> 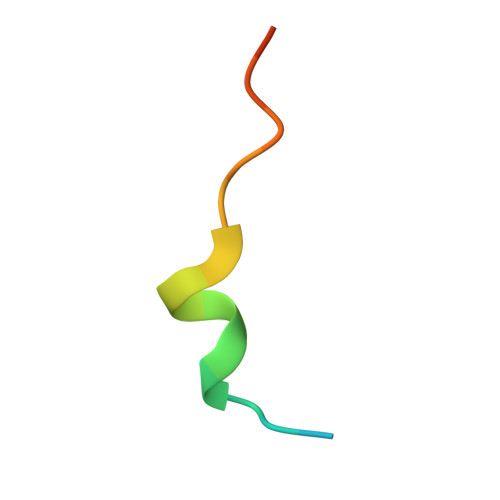MDSTDLFDVFEETPVELPTK>[2x]MAS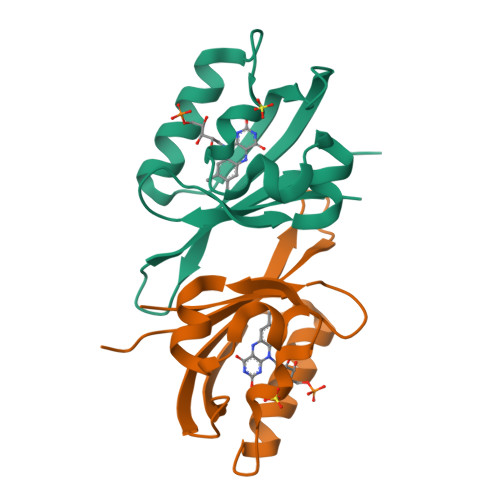GMIVTDAGADQPIVFVNRAFSTITGYAPNEVLGRNARFLQGPQTDAATVARLREAIAAARPIQERILNYRKDGQPFWNQLSISPVRDETGNVVAFVGVKTDVTAHHHHHH> ARSGSGSGSGSKLIRVGIILVLLIWGTVLLLKS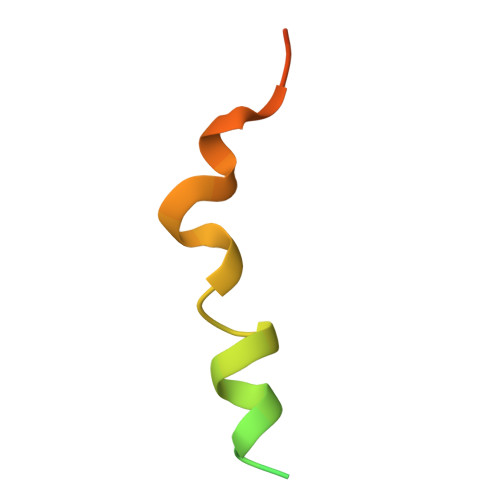IPHHHHHHH>MNTTPVHALTDIDGGIAVDPAPRLAGPPVFGGPGNDAFDLAPVRSTGREMLRFDFPGVSIGAAHYEEGPTGATVIHIPAGARTAVDARGGAVGLSGGYDFNHAICLAGGASYGLEAGAGVSGALLERLEYRTGFAEAQLVSSAVIYDFSARSTAVYPDKALGRAALEFAVPGEFPQGRAGAGMSASAGKVDWDRTEITGQGAAFRRLGDVRILAVVVPNPVGVIMDRAGTVVRGNYDAQTGVRRHPVFDYQEAFAEQVPPVTEAGNTTISAIVTNVRMSPVELNQFAKQVHSSMHRGIQPFHTDMDGDTLFAVTTDEIDLPTTPGSSR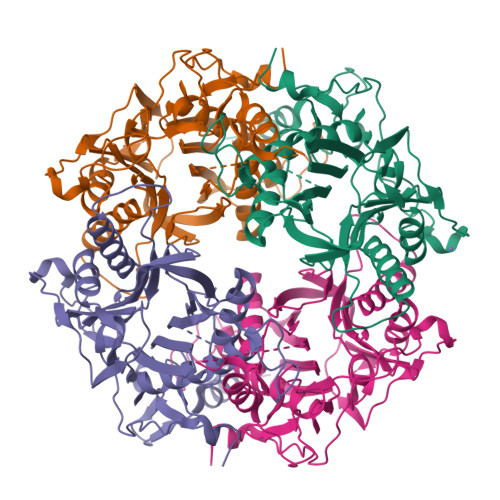GRLSVNATALGAIASEVMWDAVLEAGK[15x]>QANLMRLKSDLFNRSPMYPGPTKDDPLTVTLGFTLQDIVKVDSSTNEVDLVYYEQQRWKLNSLMWDPNEYGNITDFRTSAADIWTPDITAYSSTRPVQVLSPQIAVVTHDGSVMF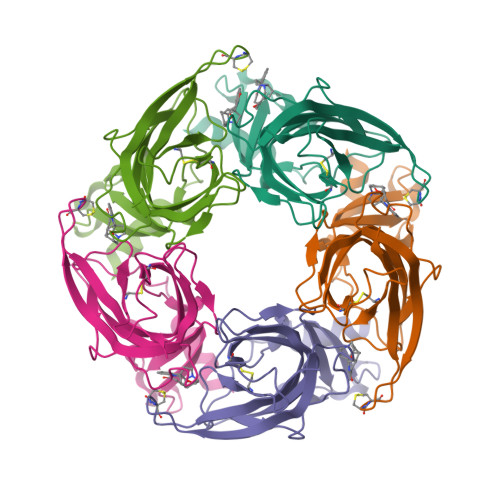IPAQRLSFMCDPTGVDSEEGVTCAVKFGSWVYSGFEIDLKTDTDQVDLSSYYASSKYEILSATQTRQVQHYSCCPEPYIDVNLVVKFRERRAGNGFFRNLFD[5x]> MSYSHSIKDCQEPDTVYYDILIPFKPNDQGFSPAIFQAQLTQPIV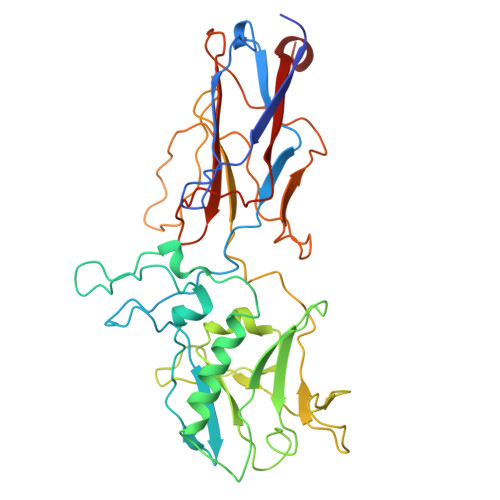HNPSEYFLSVVRFSIPTQNIPLTIPQIQPYPNTNVNNTIYSVSIGYNGTYSSQNFVQFDPSLTSPNIPAPNAPTVTSPNVEVTPYYYIYDYSTFLQMINTALENAFNEISAPVGADAPFFFYDSNTEKISLIAQAAYYDRTLTTPIEIYCNVNLFTFFDSIKHIGLGYNTPTGRDILFDVRFLGNNYYQDPETAPSYPPEFIQMQQEYPTLSNWNAVKTIQLVSNLLPINKESIPSFRNSNVGIINAQGILADFVPLVTNGPEARISIDFVATGPWRLIDMFGSVPIYMVDLYVYWTDQTGGQYLINIPPGRILTCKLVFIKKSLSKYLVSEK>[4x]ITTFTTWLLKQEQAGVIDGELTIVLSSISLACKQIASLVQRAGISNLTGLQGVANIQGEDQKKLDVISNEVFSSCLRSSGRTGIIASEEEDTPVAVEESYSGNYIVVFDPLDGSSNIDAAVSTGSIFGIYKPNEECLTDLGENPTIDEVAQNCVVNVCQPGSNLLSAGYCMYSSSVILVLS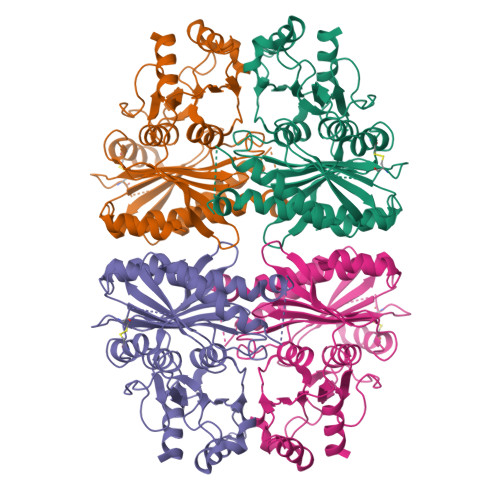VGHGVYGFTLDPLYGEFVLSHEEIKIPKSGKIYSFNEGNYALWDDKLKKYVDSLKDPGPSGKPYSARYIGSLVGDFHRTMLYGGIYGYPRDSKSKNGKLRLLYECAPMSYLAEQAGGKGSDGHQRILDIQPEQVHQRVPLYVGSTEEVEKLEKFLA> MASAPTPLAEASQIPTIPALSPLTAKQSKGNFFSSNPISSFVVDTYKQ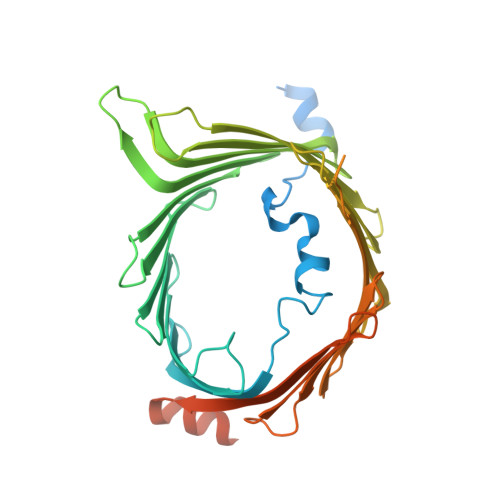LHSHRQSLELVNPGTVENLNKEVSRDVFLSQYFFTGLRADLNKAFSMNPAFQTSHTFSIGSQALPKYAFSALFANDNLFAQGNIDNDLSVSGRLNYGWDKKNISKVNLQISDGQPTMCQLEQDYQASDFSVNVKTLNPSFSEKGEFTGVAVASFLQSVTPQLALGLETLYSRTDGSAPGDAGVSYLTRYVSKKQDWIFSGQLQANGALIASLWRKVAQNVEAGIETTLQAGMVPITDPLMGTPIGIQPTVEGSTTIGAKYEYRQSVYRGTLDSNGKVACFLERKVLPTLSVLFCGEIDHFKNDTKIGCGLQFETAGNQELLMLQQGLDADGNPLQALPQLLESAGKPIPNPLLGLDST3-NITROPHENYLBORONIC 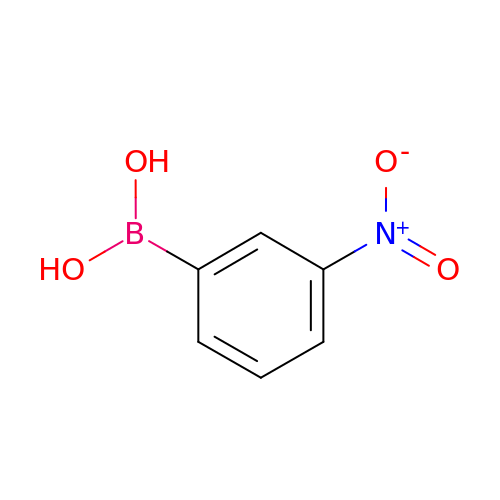ACID | C6 H6 B N O4 | ZNRGSYUVFVNSAW-UHFFFAOYSA-N> MFLKRLDVIGFKSFAERISVDFVKGVTAVVGPNGSGKSNITDAIRWVLGEQSARSLRGGKMEDIIFAGSDSRKRLNLAEVTLTLDNDDHFLPIDFHEVSVTRRVYRSGESEFLINNQPCRLKDIIDLFMDSGLGKEAFSIISQGKVEEILSSKAEDRRSIFEEAAGVLKYKTRKKKAENKLFETQDNLNRVEDILHELEGQVEPLKIQASIAKDYLEKKGPGLGTVNLGSIDEFERVNERYKFLSEQKEDLTEAKNTLFQVIEEMDEEMTKRFNDTFVQIR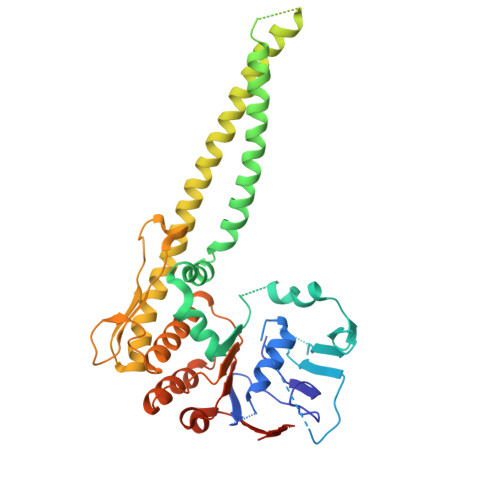SHFDQVFRSLFGGGRAELRLTDPNDLLHSGVEIIAQPPGKKLQNLNLLSGGERALTAIALLFSILKVRPVPFCVLDEVEAALDEANVFRFAQYLKKYSSDTQFIVITHRKGTMEEADVLYGVTMQESGVSKVISVKLEETKEFVQ methyl 4-({5-[(3R)-1-(hydroxyamino)-1-oxoheptan-3-yl]-1,2,4-oxadiazol-3-yl}methyl)benzoate 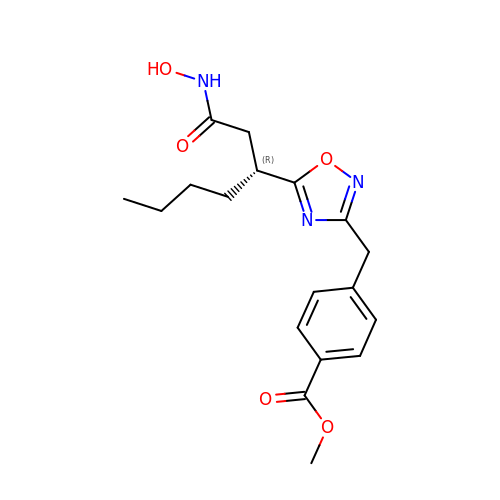| C18 H23 N3 O5 | PKBQPXFVXNPVJM-CQSZACIVSA-N>MSMQQETSHMTAAPQTNGHQIFPEIDMSAGDSSSIVRATVVQASTVFYDTPATLDKAERLLSEAAENGSQLVVFPEAF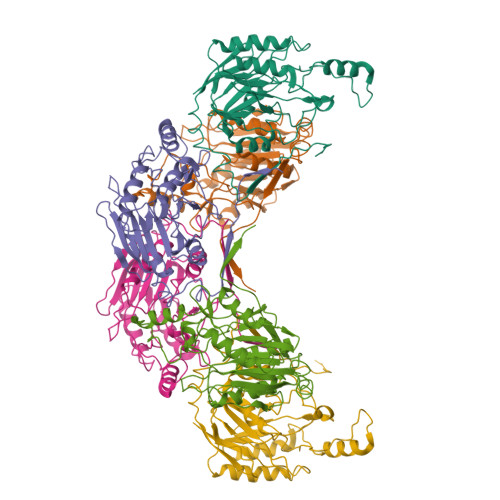IGGYPRGSTFELAIGSRTAKGRDDFRKYHASAIDVPGPEVERLALMAKKYKVYLVMGVIEREGYTLYCTVLFFDSQGLFLGKHRKLMPTALERCIWGFGDGSTIPVFDTPIGKIGAAICWENRMPSLRTAMYAKGIEIYCAPTADSRETWLASMTHIALEGGCFVLSANQFCRRKDYPSPPEYMFSGSEESLTPDSVVCAGGSSIISPLGIVLAGPNYRGEALITADLDLGDIARAKFDFDVVGHYSRPEVFSLNIREHPRKAVSFKTSKVMEDESVHHHHHH[6x]>SNAMRAQHGGKPFQQRFRVYYEDTDAGGIVYYVNYLKFMERARTERLRALGFAQSQ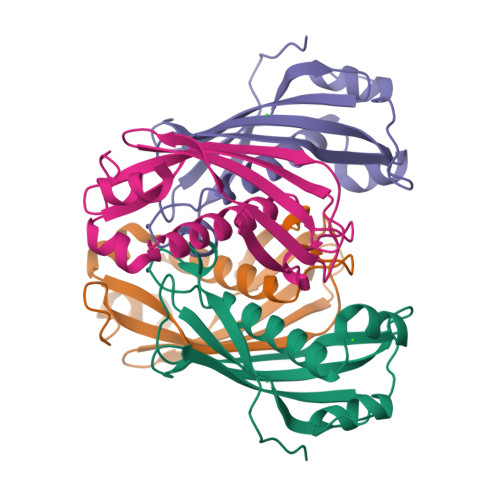LVGDNLLFVVHSAEARYHAPAKLDDELLVSAEVEELNRASLKFRQQVRRASDSVLLCEGRFLVACVRADTLKPRAIPETLRAAFAGSPDSFSAGD[2x]> GPHMRYVEIHRNLKGL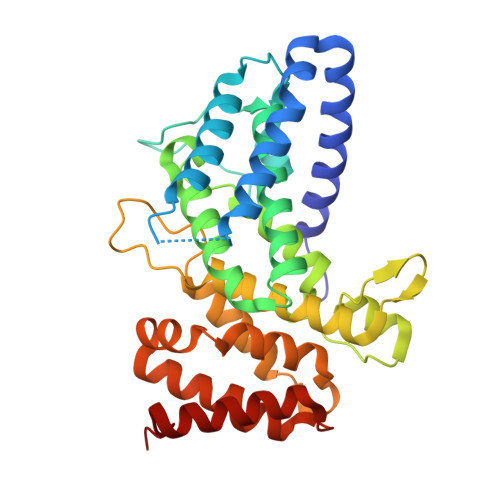RKYMAEQAKTNLKLKQRMGDMRREIRKSVGQLTTGGMAANKDKQQKIKSILTEALSNQVESALVDPNNFVVEPRKPVEGATNNDPLLPSIFVYLINIFAKAAISQFINEAGARPETADPVGICVAAILSEPDFLWRGASLIDILIAKFRIVCPVLFGYRGSEKTEQGRQRLGWWKESGQWISEQQHMDRMTGLGAGFAAISLRKFALSKKQNPYPPRFYWMAMAKIVNTPPAEISNTQCVVLKAMVQNYEAKFIEFYGSAAIAALRTALIDFPARAPHKSAAVNSLEVLAQMLKRDTGLDLG> MSNISRQAYADMFGPTVGDKVRLADTELWIEVEDDLTTYGEEVKFGGGKVIRDGMGQGQMLAADCVDLVLTNALIVDHWGIVKADIGVKDGRIFAIGKAGNPDIQPNVTIPIGAAT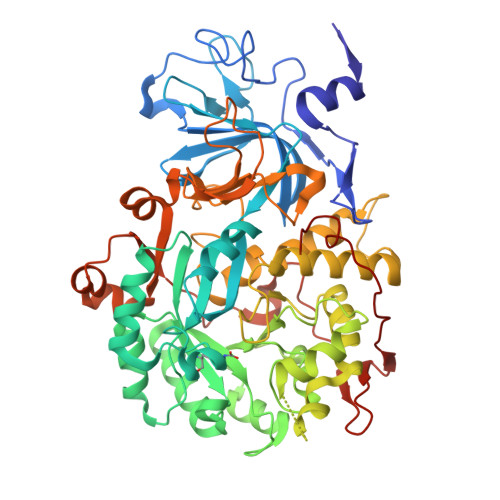EVIAAEGKIVTAGGIDTHIHWICPQQAEEALVSGVTTMVGGGTGPAAGTHATTCTPGPWYISRMLQAADSLPVNIGLLGKGNVSQPDALREQVAAGVIGLKIHEDWGATPAAIDCALTVADEMDIQVALHSDTLNESGFVEDTLAAIGGRTIHTFHTEGAGGGHAPDIITACAHPNILPSSTNPTLPYTLNTIDEHLDMLMVCQHLDPDIAEDVAFAESRIRRETIAAEDVLHDLGAFSLTSSDSQAMGRVGEVILRTWQVAHRMKVQRGALAEETGDNDNFRVKRYIAKYTINPALTHGIAHEVGSIEVGKLADLVVWSPAFFGVKPATVIKGGMIAIAPMGDINASIPTPQPVHYRPMFGALGSARHHCRLTFLSQAAAANGVAERLNLRSAIAVVKGCRTVQKADMVHNSLQPNITVDAQTYEVRVDGELITSEPADVLPMAQRYFLF>[2x]TPLRDEQEEASTKLMQWLRGVGDAPPSASMSDENASVSSANELIFCQVDGIDYAFYNTKEKAMLGYMRFKPYQKRSMKQAKVHPLKLLVQFGEFNVETLAVGEEKEVHSVLRVGDM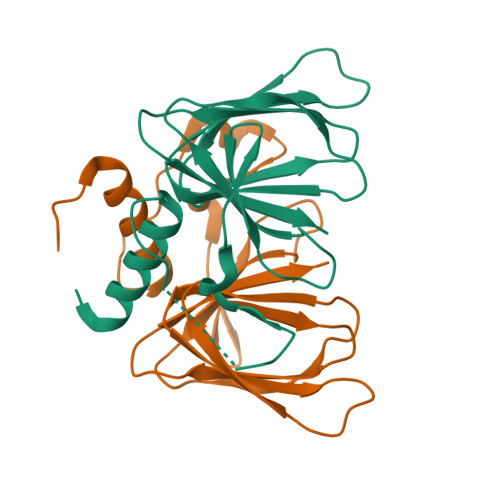IEIDRGTRYSIQNAIDKVSVLMCIRS> TEFKAGSAKKGATLFKTRCLQCHTVEKGGPHKVGPNLHGIFGRHSGQAEGYSYTDAIIKKNVLWDENNMSE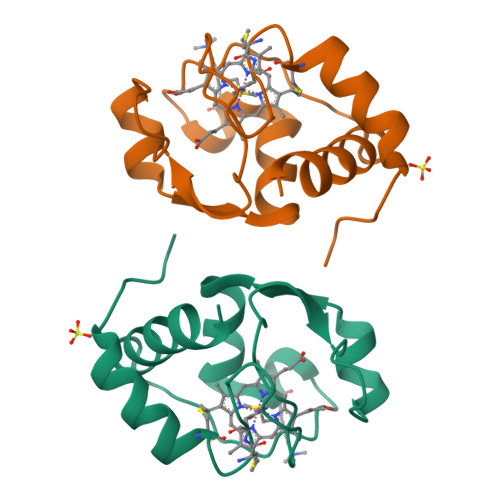YLTNPKKYIPGTKMASGGLKKEKDRNDLITYLKKAAE> MDVLRTPDERFEGLADWSFAPHYTEVTDADGTALRIHHVDEGPKDQRPILLMHGEPSWAYLYRKVIAELVAKGHRVVAPDLVGFGRSDKPAKRTDYTYERHVAWMSAWLEQNDLKDIVLFCQDWGGLIGLRLVAAFPERFSAVVVSNTGLPIGVGKSEGFEAWLNFSQNTPELPVGFILNGGTARDLSDAERSAYDAPFPDESYKEGARIFPALVPITPEHASVEENKAAWAVLETFDKPFVTAFSDADPITRGGEAMFLARVPG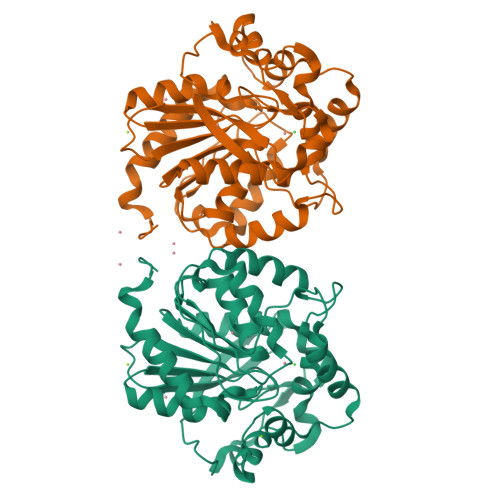TKNVAHTTLKGGHFVQEDSPVEIAALLDGLVAGLPQAHHHHHH>EVAAMDFTDKLIISRPLYISDNADPKCGYCNGKKDSSHKFASPGWSDFYKGDEDKVELQSSTVGFNSELVNAETYDKLCNLGFRRSGSFMYKTDMLRNCCRLYTIRTNEKYLTMSKELKTSLKRFKKKITSPEFKPQPKYVSWIDELCDYEPKSTSFKAVFEPAEFTDEKYDLYVRYQHYIHSDEDNTPSQFESFLCDTPFTDSEITGTEKEWEQLNNWHNLQPGERVTKNGPAHECYYHNGKLIALSVLDFLPSGVSSVYFIWDPDYYDWSLGKVSALRELALVSKIGRPYYYLGYYID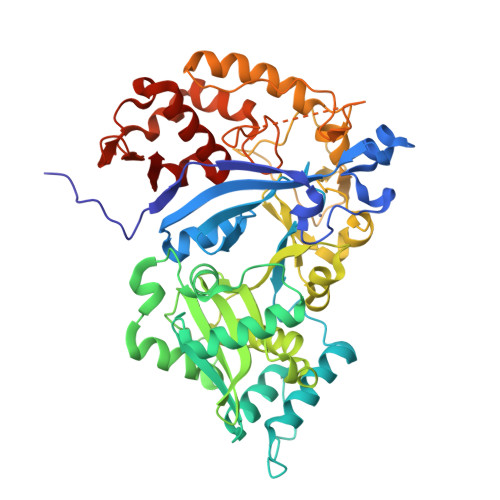DCPKMNYKAKFGGEILDVCNQKYVPLSKIHQIIKHNELFVGLNSTVASPDSEILITSASDKINFDEPFINAVDDIYGPNGNASQNAITSVAKLRKYGINYSPDLQRSIYKEIPNDGNSTSSASSDKKDVYRIPNVVPGLVPLMEIVSLFESGKMNELNNNVVLFDTKINALRIVRDFISEKPEIKTVITDVIRLIGLDNTKKAIIII[2x]>[2x]MPEFRMPEFEKSKLHIAMYPWVAMGHITPFIHLANELAKRGHSISILLPQKALLQLGHNNLYPDLIKFHLVTVPQVDGLPPGAETASDIDITAKNPLAIAFDATSEQVETLLHSLKPDIVFYDFADWIPKLA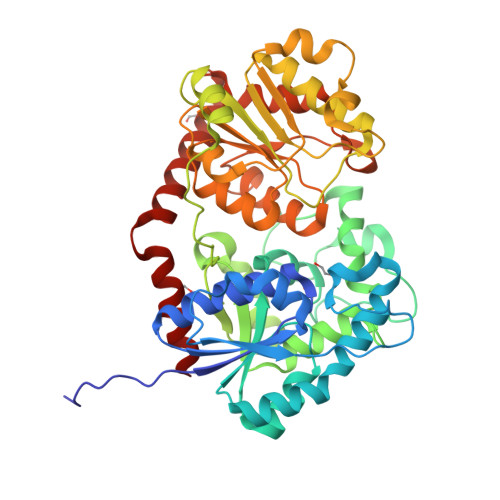AQIGFKTVCYNVICASVMAIGIVPARHIPKDRPLTEQELMEPPRGYPSSTVVLRGQEALTLSFIGMDYGATKFDVRITASMQGCDAIGIRTCRELEGPMCDYLSAQYNKPVFLSGPVLPETPKGPLEEKWDSWLNKFKPKSVVYCAFGSQMILQKNQFQELVLGFEMTGLPFFIALSKPHGADSVEEALPDGFLERVGDRGVVHGGWVQQTQILNHPSVGCFVSHCGFGSMWESLLSESQIVLVPRLADQILNTRLLAEELKVAVEVERGDMGWFSKEDLSKAIKSVMDEDSEVGKLVKQNHAKWKETLVSPGFMDNYIDNFIQQLYQ>[2x]MNGPIIMTREERMKIVHEIKERILDKYGDDVKAIGVYGSLGRQTDGPYSDIEMMCVMSTEEAEFSHEWTTGEWKVEVNFYSEEILLDYASQVESDWPLTHGQFFSILPIYDSGGYLEKVYQTAKSVEAQTFHDAICALIVEELFEYAGKWRNIRVQGPTTFLPSLTVQVAMAGAMLIGLHHRICYTTSASVLTEAVKQSDLP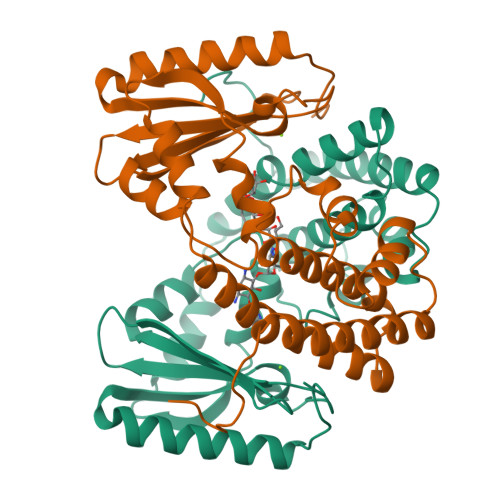SGYDHLCQFVMSGQLSDSEKLLESLENFWNGIQEWTERHGYIVDVSKRIPF> MDETGKYLVLALYDYQEKSPREVTMKKGDILTLLNSTNKDWWKVEVNGRQG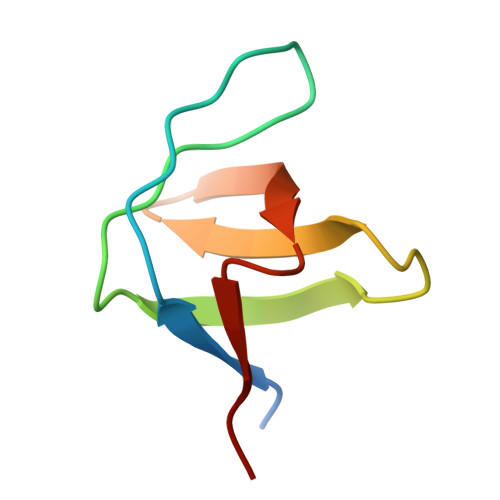FVPAAYVKYLD>ASLTEIEHLVQSVCKSYRETCQLRLEDLLRQRSNIFSREEVTGYQRKSMWEMWERCAHHLTEAIQYVVEFAKRLSGFMELCQNDQIVLLKAGAMEVVLVRMCRAYNADNRTVFFEGKYGGMELFRALGCSELISSIFDFSHSLSALH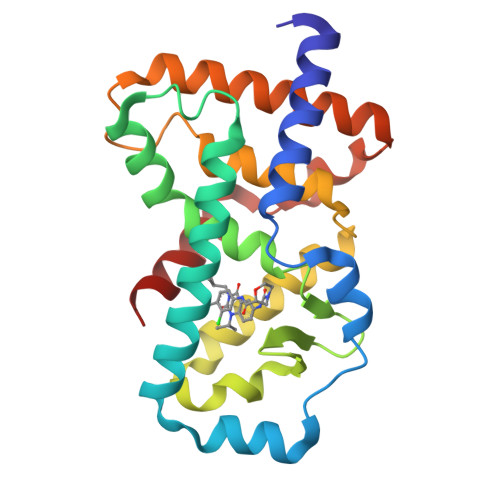FSEDEIALYTALVLINAHRPGLQEKRKVEQLQYNLELAFHHHLCKTHRQSILAKLPPKGKLRSLCSQHVER[2x]> MTEHSLWRFSRALHRALNDRQTEELATIIDDNIDWAIYGPIDMFPFFGARQGKAAVLEVCRQIADSVRIYRYHRESVML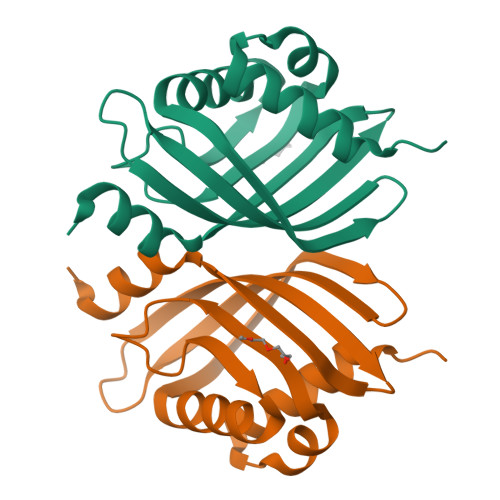GIDSAASMVRYSLTAAGTNRPISVRMALFTQFQNGRLTNLRMVLDTFDLVEQALGRPIHLPKIA> MLKCSLCYLASKVTAGNAKNQAGHPRRKAKLFHVVPGTPVTPFEKLKEQRRRFG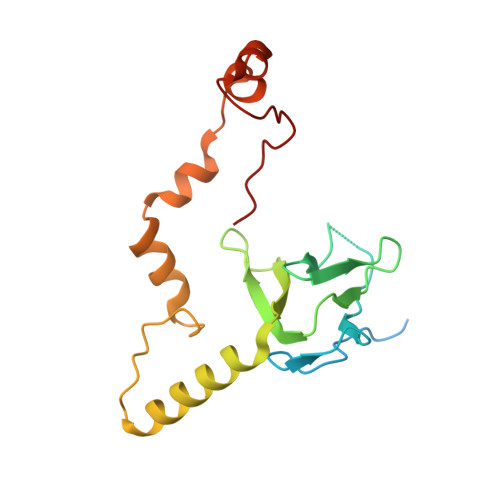QDRHSRLPEYRPGNNVRMDPNTYTLYATKKGVMTIRESRINPKYKWLDVEPDIQKVYRSRELRRALQEREMASMAVGENSNYRVELDLLLEPDWRERVMHVPKATERFKDPNLFTRGVVNELSPLDRYSYT> MTSKHFISKKEAKRIWEQMSRYGIDITGESLEVAAQKSASAYYIGGKPMVFQAGDLIPSVYLLNYRNPSRNIVT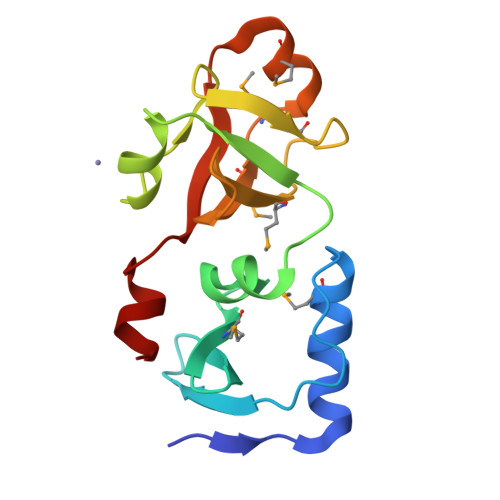VDEGAEPHILNGSDLFAPGIVSMDDSIRKGDMIFVKSSKGYFIAVGMAEMDAGEVMATKRGKAARIIHFPGDELIRAFP>[4x]GPMSKKLSVQEIILTLQKFWSDQGCMLMQSYDTEKGAGTMSPYTFLRAIGPEPWNAAYVEPSRRPADGRYGENPNRLYQHHQFQVVMKPSPENVQDLYLQSLEKLGINPLEHDIRFVEDNWENPSMGCAGVGWEVWLDGMEISQFTYFQQVGGLEVDPVTSEITYGLERLSSYIQDVNSVFDLEWGDGVKYGDIFLEPEFENSKYAFEDSNEELLLMLFDEYEKEAKRQIKNGLVH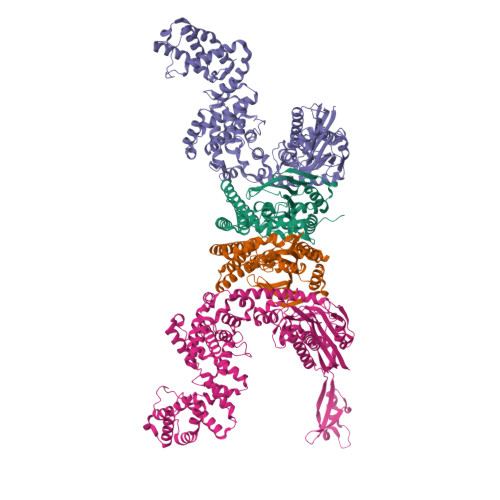PAYDYCLKCSHTFNLMDARGMVSVTERAGYLDRIRNMAKSIAKEFVAQREKRGFPLLKHAQEETK;>MAKTYLLEIGLEEMPAHVVTPSVLQLKERMIKFLKDARLDFEDVKTFSTPRRLTVQVLGLADKQADVKKEVRGPAKKIAQDADGNWTKAAIGFSKGQGASTDDIVFKDVKGTPYVFVQTFTAGKTAAEVLTGGIKDVITKMNFPTMMKWSTYSFKYIRPIRWIVSLLDDEVVPVQILDVAAGRVSRGHRFLGHDVEIATAADYEADLASVQVVADAAKRKATIREQIAALANERDWQIKVNEDLLEEVNNLVEYPTAFAGDFDTKYLTIPDEVLITSMRDHQRFFYVTDAEDNLLPHFVSVRNGNTDHLENVALGNQKVLTARLEDAAFFYHEDQQHSIQEYVERLKKVSFHDKIGTMYEKMQRVMIISDFLADRFGLTETEKNQLHRAAQIYKFDLVTGMVGEFPELQGVMGDKYAVLKGEDPAVGQAIREHYMPISADGDLPKSKVGAVLAIADKVDSITSFFAVGLTPSGSNDPFALRRQAFGIVRIVREQGWDFPIRQLEADIQKELVAHDATYNLDFEKQTAPVADFLTDRVKQWFNNRKIRYDIVDTVIKGSRQDIREMFKAADVLNAHQDDPQFKDTIEAFTRLLRITAKAKLAADDLTVDPSLFENEAEQHLYDAVLELQKQFTPAMSMEDRFKALAALRPLIVDYFEQTMVMSKDEKVRDNHLKQLLTIAQMINVMGDLNQLIVK[4x]>MSVLQVLHIPDERLRKVAKPVEEVNAEIQRIVDDMFETMYAEEGIGLAATQVDIHQRIIVIDVSENRDERLVLINPELLEKSGETGIEEGCLSIPEQRALVPRAEKVKIR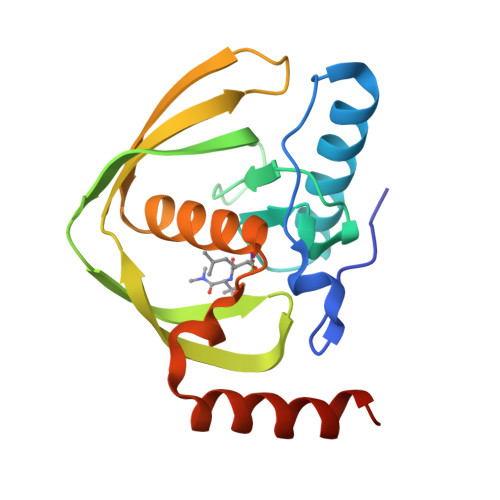ALDRDGKPFELEADGLLAICIQHEMDHLVGKLFMDYLSPLKQQRIRQKVEKLDRLKARA[3x]>LPDLKIEKLEEGVFVHTSFEEVNGWGVVTKHGLVVLVNTDAYLIDTPFTATDTEKLVNWFVERGYEIKGTISSHFHSDSTGGIEWLNSQSIPTYASELTNELLKKSGKVQAKYSFSEVSYWLVKNKIEVFYPGPGHTQDNLVVWLPESKILFGGCFIKPHGLGNLGDANLEAWPKSAKILMSKYGKAKLV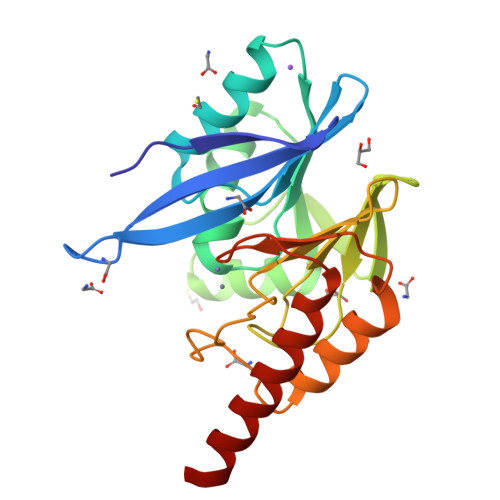VSSHSEKGDASLMKRTWEQALKGLKESKKT[4x]> VVGGEDAKPGQFPWQVVLNGKVDAFCGGS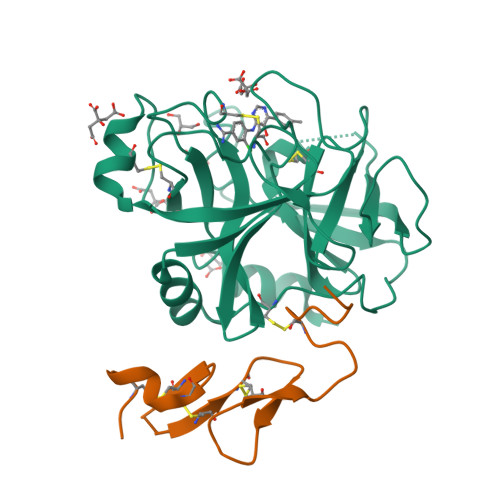IVNEKWIVTAAHCVETGVKITVVAGEHNIEETEHTEQKRNVIRIIPHHNYNAAINKYNHDIALLELDEPLVLNSYVTPICIADKEYTNIFLKFGSGYVSGWGRVFHKGASALVLQYLRVPLVDRATCLRSTKFTIYNNMFCAGFHEGGRDSCQGDSGGPHVTEVEGTSFLTGIISWGEECAMKGKYGIYTKVSRYVNWIKEKTKLT;> MDVTCNIKNGRCEQFCKNSADNKVVCSCTEGYRLAENQKSCEPAVPFPCGRVSVSQTSKLTR>[3x]HHHHHHMVLIPNKPAPEFHGCAVIDGDFKEINLKDYSGKYVVLFFYPADFTFVCPTEIIA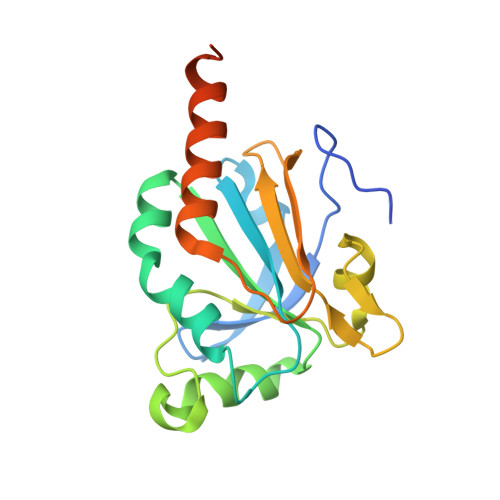FSDEVDQFKSRNCQVIACSTDSKYSHLAWTKQDRKSGGLGDMRIPLLADPTKSIARAYGVLDEEEGNAFRGLFIIDPKGILRQITVNDKPVGRSVDETLRLLDAFQFVEKYGEVCPVNWKRGQHGIKVNH> AFQGQAPSFKAEAVFGDNTFGEVSLSDFIGKKYVLLYFYPLDFTFVCPSEIIALDKALDSFKERNVELLGCSVDSKFTHLAWKKTPLSQGGIGNIKHTLISD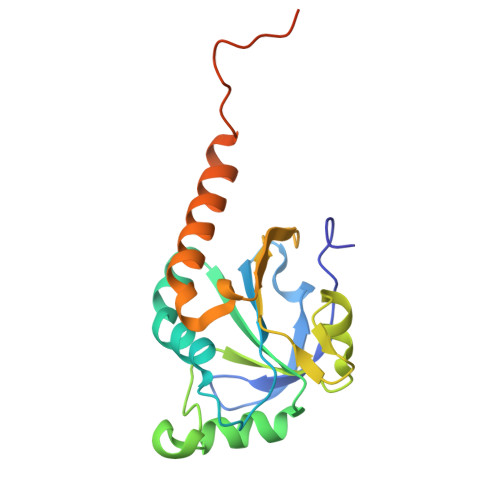ISKSIARSYDVLFNESVALRAFVLIDKQGVVQHLLVNNLALGRSVDEILRLIDALQHHEKYGDVCPANWQKGKESMKPSEEGVAKYLSNL> SNAMVRVDQNLFNEVMYLLDELSQDITVPKNVRKVAQDSKAKLSQENESLDLRCATVLSMLDEM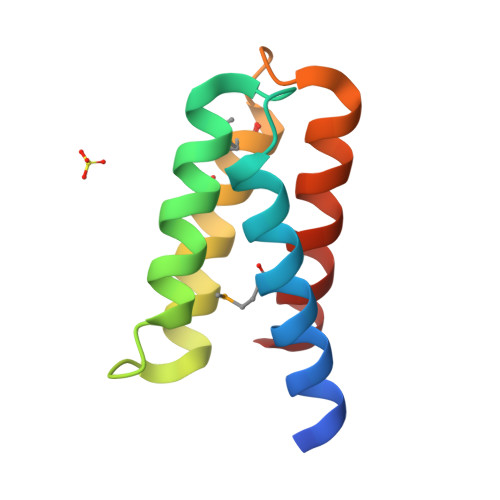ANDPNVPAHGRTDLYTIISKLEALS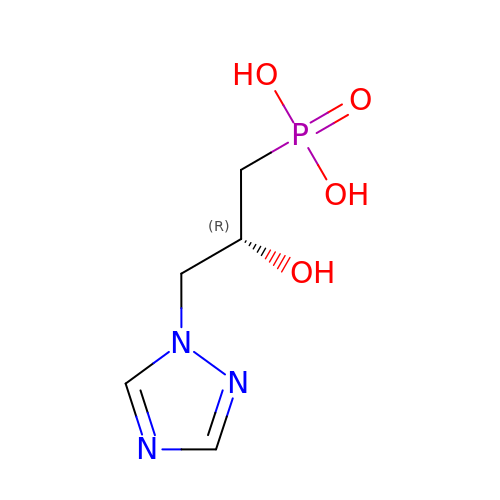[(2R)-2-hydroxy-3-(1H-1,2,4-triazol-1-yl)propyl]phosphonic acid | C5 H10 N3 O4 P | ZXKJPBBOMRHTCH-RXMQYKEDSA-N(1~{S},2~{R},3~{S},4~{R},5~{R},6~{R})-5-[[4-[4-[(12~{R})-2,2-bis(fluoranyl)-4,6,10,12-tetramethyl-1,3-diaza-2$l^{4}-boratricyclo[7.3.0.0^{3,7}]dodeca-4,6,9-trien-8-yl]butyl]-1,2,3-triazol-1-yl]methyl]-7-oxabicyclo[4.1.0]heptane-2,3,4-triol 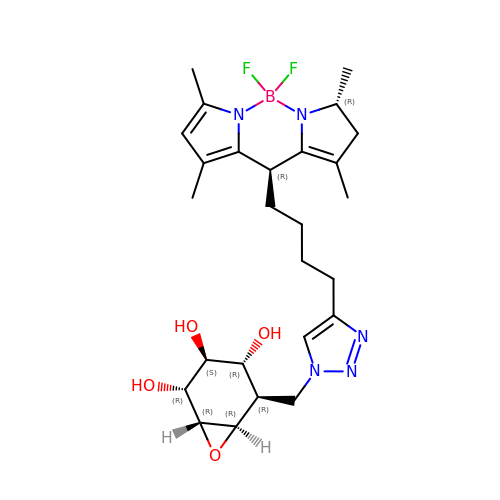| C26 H37 B F2 N5 O4 | AJWVMTKRGUGWOR-QHKJSSTCSA-N> NEKLAKKKIVSIDAGRKYFSPEQLKEIIDKAKHYGYTDLHLLVGNDGLRFMLDDMSITANGKTYASDDVKRAIEKGTNDYYNDPNGNHLTESQMTDLINYAKDKGIGLIPTVNSPGHMDAILNAMKELGIQNPNFSYFGKKSARTVDLDNEQAVAFTKALIDKYAAYFAKKTEIFNIGLDEYANDATDAKGWSVLQADKYYPNEGYPVKGYEKFIAYANDLARIVKSHGLKPMAFNDGIYYNSDTSFGSFDKDIIVSMWTGGWGGYDVASSKLLAEKGHQILNTNDAWYYVLGRNADGQGGGNLDQGLNGIKNTPITSVPKTEGADIPIIGGMVAAWADTPSAR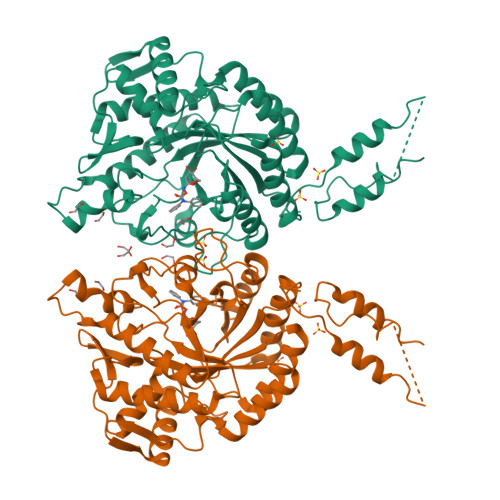YSPSRLFKLMRHFANANAEYFAADYESAEQALNEVPKDLNRYTAESVTAVKEAEKAIRSLDSNLSRAQQDTIDQAIAKLQETVNNLTLTP> SLLTCGGCQQNIGDRYFLKAIDQYWHEDCLSCDLCGCRLGEVGRRLYYK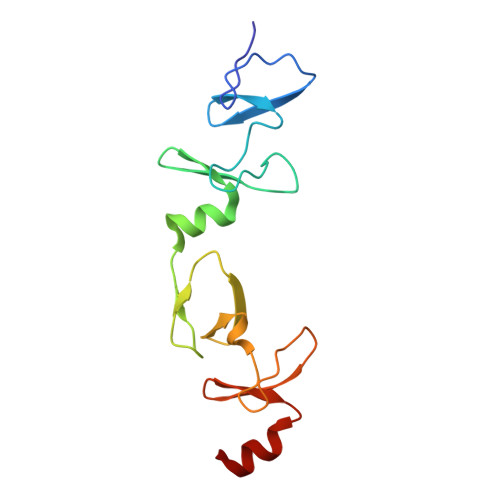LGRKLCRRDYLRLFGQDGLCASCDKRIRAYEMTMRVKDKVYHLECFKCAACQKHFCVGDRYLLINSDIVCEQDIYEWTKING>[2x]APQQINDIVHRTITPLIEQQKIPGMAVAVIYQGKPYYFTWGYADIAKKQPVTQQTLFELGSVSKTFTGVLGGDAIARGEIKLSDPTTKYWPELTAKQWNGI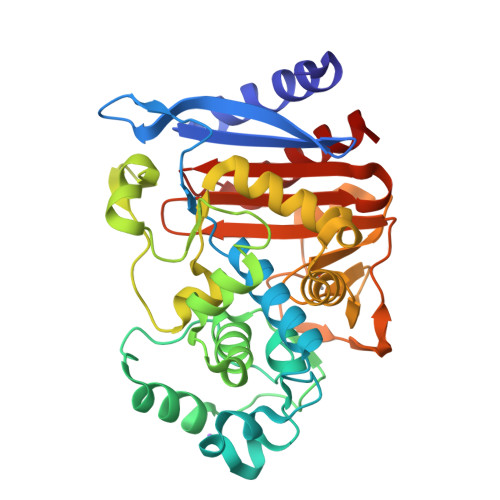TLLHLATYTAGGLPLQVPDEVKSSSDLLRFYQNWQPAWAPGTQRLYANSSIGLFGALAVKPSGLSFEQAMKTRVFQPLKLNHTWINVPSAEEKNYAWGYREGKAVHVSPRALDAEAYGVKSTIEDMARWVQSNLKPLDINEKTLQQGIQLAQSRYWQTGDMYQGLGWEMLDWPVNPDIIINNKIALAARPVKPITPPTPAVRASWVHKTGATGGFGSYVAFIPEKELGIVMLANKNYPNPARVAAAWQILNALQ> NTGDNSVSTTKTSTRIVGGTNSSWGEWPWQVSLQVKLTAQRHLCGGSLIGHQWVLTA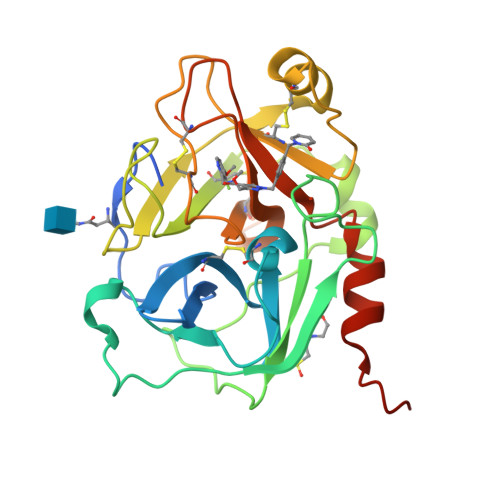AHCFDGLPLQDVWRIYSGILNLSDITKDTPFSQIKEIIIHQNYKVSEGNHDIALIKLQAPLNYTEFQKPISLPSKGDTSTIYTNCWVTGWGFSKEKGEIQNILQKVNIPLVTNEECQKRYQDYKITQRMVCAGYKEGGKDACKGDSGGPLVCKHNGMWRLVGITSWGEGCARREQPGVYTKVAEYMDWILEKTQSSDGKAQMQSPA> VTAVVQRVEIHKLRQGENLILGFSIGGGIDQDPSQNPFSEDKTDKGIYVTRVSEGGPAEIAGLQIGDKIMQVNGWDMTMVTHDQARKR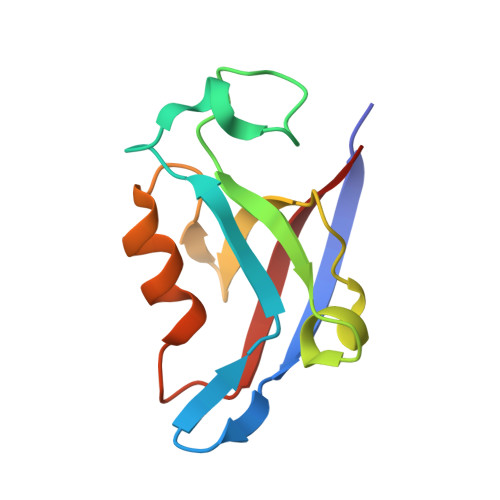LTKRSEEVVRLLVTRQ>[2x]MAHHHHHHVDDDDKMVHHDGFQTVKATIDWEHPMFKLYEKAKRNGKWNPADIDFSQDQKDFASLTSEEKISALPLVAGFSAGEEAVTLDILPMAHALARQGRLEDVLFLTTFMHDEAKHVEMFSRWQQAVGIGQMDLSVFHNDHYKRIFYEALPEAMNRLYADDSPEAVIRAATVFNMIVEGTLAESGYYTFRQIYKKAGLFPGLLQGIDYLNMDEGRHIQFGIYTIQRIVNEDERYYELFIRYMDELWPHVIGYVDYLTELGKRQQQLARTYALEIDYDLLRHYVIKQFNLRKKQISRTKRVDVVEGLEKTAAES

A related group of proteins with a similar Mn/Fe cofactor is termed R2-like ligand-binding oxidases (R2lox). Following O2 activation, their cofactor catalyzes a two-electron redox reaction which results in the formation of a tyrosine–valine ether cross-link in the protein. The tyrosine and valine residues are conserved in the R2lox group, and the cross-link was observed in both R2lox proteins that have been structurally characterized. Both proteins also comprise a hydrophobic channel leading to the metal cofactor wherein a long-chain fatty acid molecule is found, which coordinates at the Mn/Fe ions of the cofactor. The mixed-metal cofactor in R2lox self-assembles with the manganese ion in metal-binding site 1 and the iron ion in site 2 if both MnII and FeII are available.

The valine was changed to alanine, isoleucine, or leucine (V72A/I/L), and the tyrosine was changed to phenylalanine (Y162F). The mutation of the cross-link tyrosine to a phenylalanine was found to have little effect on the active site and global protein structure of R2lox, although the hydrogen bond to the carbonyl oxygen of V72 is missing in the reduced state and the cross-link cannot be formed upon oxidation. Interestingly, in the structure of the aerobically reconstituted protein, only one of the two subunits of the dimer in the asymmetric unit of the crystals is in the oxidized state conformation. Very weak difference density for the oxidized conformation in the other subunit suggested that the reduced state conformation was present in at least 90% of this molecule (not shown). This asymmetric behavior might be caused by different packing interactions of the two molecules in the crystal. It should be noted, however, that other mutants that crystallized in the same space group (V72A/L-R2lox) did not display large differences between the two subunits. It appears, therefore, that the asymmetry is caused by the Y162F mutation, either because O2 activation is partially impaired in Y162F-R2lox, or because one subunit is more sensitive to X-ray photoreduction during diffraction data collection, an effect previously observed in a related class Ib R2 protein. No impairment of O2 reduction could be observed in Y162F-R2lox in solution. This suggests that enhanced sensitivity to photoreduction was the reason for the reduced state conformation that is prevalent in one of the two subunits of the oxidized state Y162F-R2lox crystal structure (see above). Like the wild-type, the Y162F and V72A mutants assemble mostly (Mn/Fe)III/FeIII cofactors, suggesting that in the absence of cross-link formation, putative metal(IV) species formed after full O2 reduction are partially reduced by external electron sources.> MVDATRVPMDERFRTLKKKLEEGMVFTEYEQIP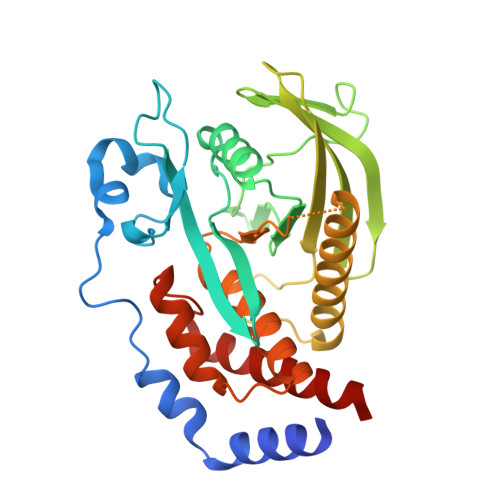KKKANGIFSTAALPENAERSRIREVVPYEENRVELIPTKENNTGYINASHIKVVVGGAEWHYIATQGPLPHTCHDFWQMVWEQGVNVIAMVTAEEEGGRTKSHRYWPKLGSKHSSATYGKFKVTTKFRTDSVCYATTGLKVKHLLSGQERTVWHLQYTDWPDHGCPEDVQGFLSYLEEIQSVRRHTNSMLEGTKNRHPPIVVHCSAGVGRTGVLILSELMIYCLEHNEKVEVPMMLRLLREQRMFMIQTIAQYKFVYQVLIQFLQNSRLI> 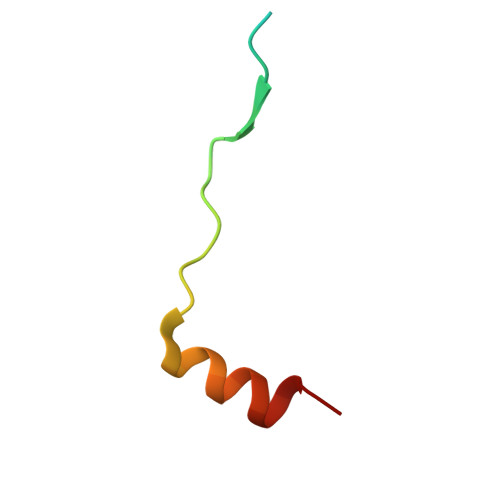MWFPYDGSKLPLRPKRSPPVISEEAAEDVKQYLTI> GAGCAGACGAG;> ACCGC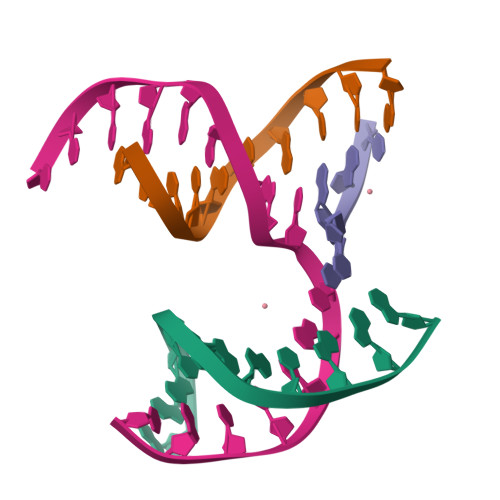ACTCA;> CTGGT;> TCTGAGTGCCGTCTGC> GCPRILIRCKQDSDCLAGCVCG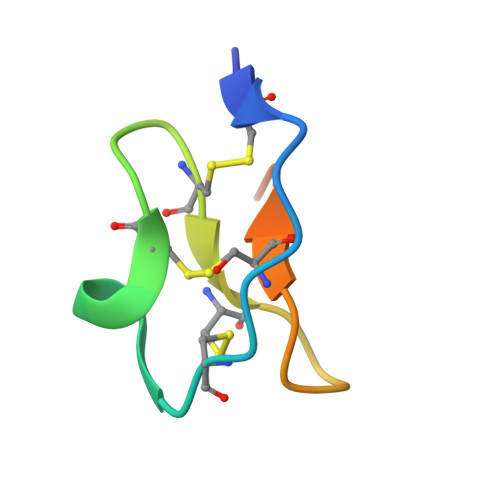PNGFCGSPHHHHHH>[2x]GAINLYSSRHYDTDQALYDSFTKKTGLKVNLIEGKGDKLIERIKSEGANSPADVFMTVDAGRLWRAQEAGILQPISSSTLNNKIPANLRSPEKLWFGFSKRARVIMYNKNKVQPSELSTYEDLAQNKWKGKIVIRSSSNIYNQSLIASLIEIHGMSDAEGWAKGFVRNFARPPEGNDTAQI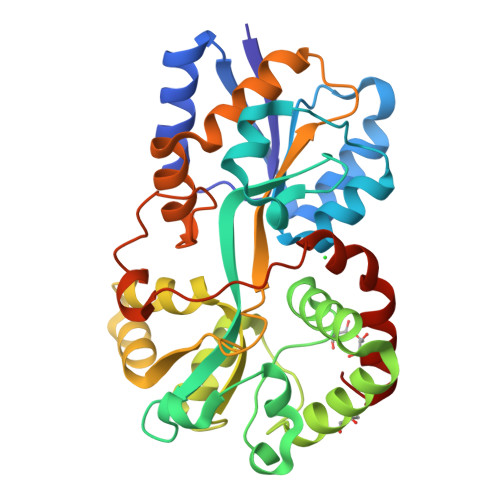KAVAAGIGDIGLANSYYLARLKRSSKPEDQAVADKVGMFFPNQNGRGTHVNISGGGVVKNAPNKEGAIKFLEYLVSPEAQKIFSEGNNEYPVVAGVPIASVLKPFGSFKNDSTNVSVYGKLNADAIKLMDRVGWKLE> ALTAKHRPSVVWLHNAECTGCTEAAIRTIKPYIDALILDTISLDYQETIMAAAGEAAEAALHQALEGKDGYYLVVEGGLPTIDGGQWGMVAGHPMIETTKKAAAKAKGIICIGTCSAYGGVQKAKPNPSQAKGVSEALGVKTINIPGCPPNPINFVGAVVHVLTKGIPDLDENGRPKLFYGELVHDNCPRLPHFEASEFAPSFDSEEAKKGFCLYELGCKGPVTYNNCPKVLFNQ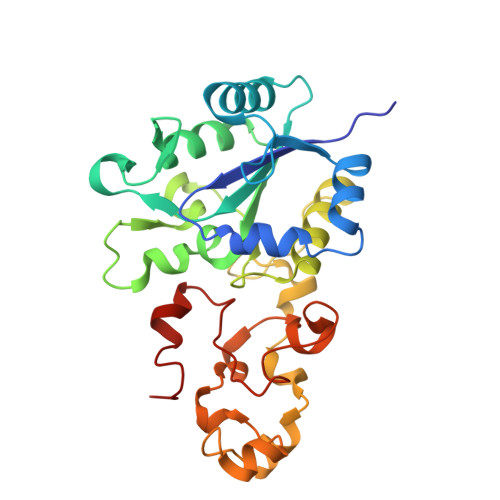VNWPVQAGHPCLGCSEPDFWDTMTPFYEQG> MSQSHLDDLFAYV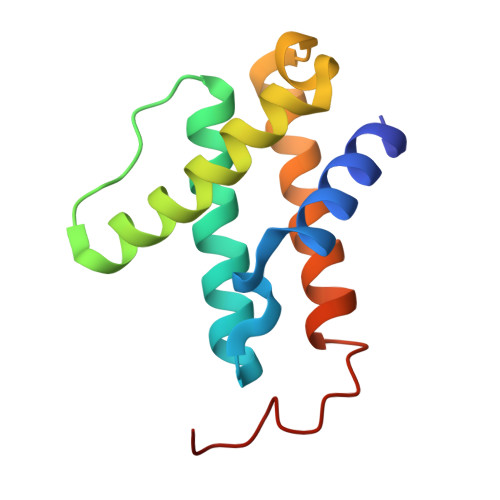EERCLWQFFSRTWDREENIEGVLNQVGRLLTGQEPLRGTPQERLFYADALAMANDVRERFPWASQVNKEEIEFLLDGLKSRLVDVTITRSTNRELNHHLY> MEEKAKSIDQATLQLLDKAKQDGVETVWDRKADMKVQCGFGSAGVCCRNCSMGPCRVSPVPGKGVERGICGATADVIVSRNFARMVAAGTAAHSDHGRSIALSLYHTSKDGDIKVKDENKLKEVAKSFNVETEGRDIYDIAHDVAKEGLSNYGKQLGEVTLPPSLPEKRKELWRKLGVYPRAVDREIAAVMHSTHIGCNADAEAMIKMSMRCSLTDGWMGSFMGTEFSDIMFGTPHSIDTEANLGVLEKNSVNVVLHGHEPLLSEMVVEAASDPELVELAKSVGADGINLCGMCCTGNEVSMRHGIKIAGNFMQQELAVVTGAVDGLIVDVQCIMPALAKLSKSYHTKFITTSPKAHITDSIYMEFDEENPLDSAKKILKEAILNFKNRDQSKVMIPELKCKAILGYSVEEIINKLDKVVNTQIGPMQTVKPLADVLVSGVLR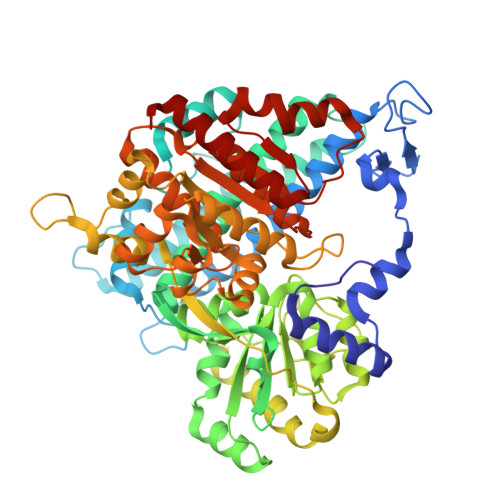GAAAVVGCNNPKVVQDSAHIETIKGLIKNDVIVVVTGCAAQAAAKYGLLQKEAAEKYAGPGLATVCKLVDIPPVLHMGSCVDISRILDLVGRVANLLGVDMSDLPVAGVAPEWMSEKAVAIGTYVVTSGIDTWLGVAPPVTGGPEVVDILTNKMEDWVGAKFFIETDPHKAVEQIVNRMNEKRKKLGI> AVSKVYARSVYDSRGNPTVEVELTTEKGVFRSIVPSGASTGVHEALEMRDGDKSKWMGKGVLHAVKNVNDVIAPAFVKANIDVSDQKAVDDFLISLDGTANKSKLGANAILGVSLAASRAAAAEKNVPLYKHLADLSKSKTSPYVLPVPFLNVLNGGSHAGGALALQEFMIAPTGAKTFAEALRIGSEVYHNLKSLTKKRYGASAGNVGDEGGVAPNIQTAEEALDLIVDAIKAAGHDGKVKIGLDCASSEFFKDGKYDLDFKNPNSDKSKWLTGPQLADLYHSLMKRYPIVSIEDPFAEDDWEAWSHFFKTAGIQIVADDLTVTNPKRIATAIEKKAADALLLKVNQIGTLSESIKAAQDSFAAGWGVMVSHRSGETEDTFIA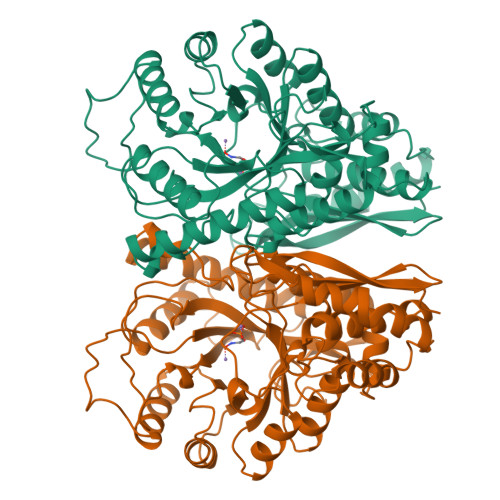DLVVGLRTGQIKTGAPARSERLAKLNQLLRIEEELGDNAVFAGENFHHGDKL>[10x]MAHHHHHHVDDDDKMRTPTVAPPAPVYRD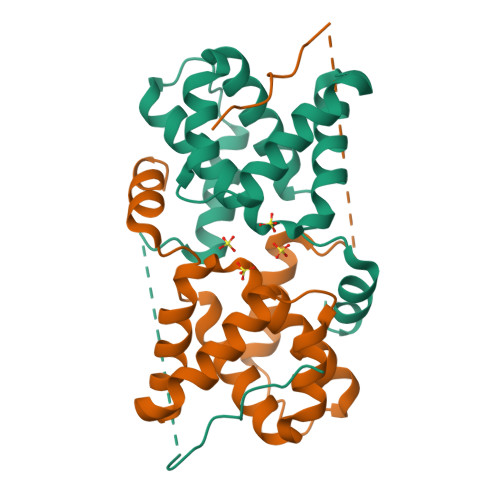HSEKKELPQDEQQDGPKITLLTLIKTAEHWARQDIRTIEDSKLRALLTLCAVMTRKFSKSQLSLLCETHLRREGLGQDQAEPVLEVYQRLHSDKGGSFEAALWQQWDRQSLIMFITAFLNIALQLPCESSAVVVSGLRTLVPQSDNEEASTNPGTCSWSDEGTP>HHHHHHGSGGDYFPVISVDLQSGRRVVSVEYIRGDGPPRIPYSMVGPCCVFLMHHRPSHEVRLRFSDFYNVGEFPYRVGLGDFASNVAPPPAKPFQRLIDLIGHMTLSDFTRFPNLKEAISWPLGEPSLAFFDLSSTRVHRNDDIRRDQIATLAMRSCKITNDLEDSFVGLHRMIVTEAILRGIDLCLLPGFDLMYEVAHVQCVRLLQAAKEDISNAVVPNSALIALMEESLMLRSSLPSMMGRNNWIPVVPPIPDVEMESEE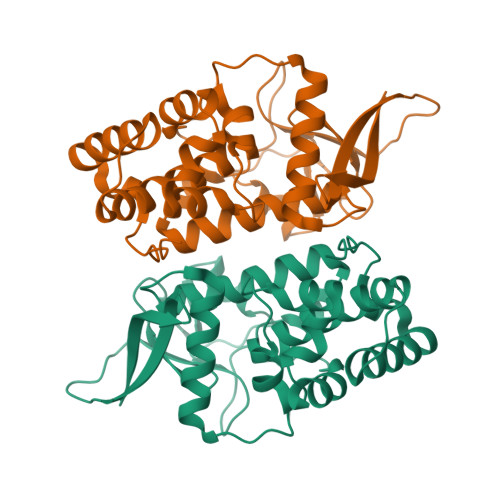ESDDDGFVEVD[2x]>AHHHHHHGSPLPPDITFDSLALIKMHSQSMKK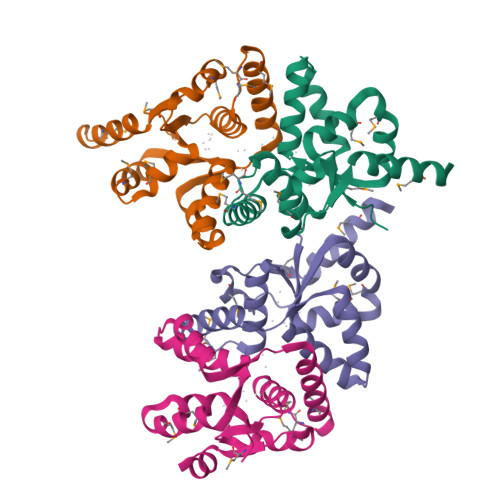ILEITLAKFTVNLSIVTVYRYLTVRAYLKKNIELELDVLKDIYNIVPLNEEIAIKAAQIEADLMRKGMMPDIEDVLTAATAIYTKSLLITDDSKRYEPMRRFGLDTMPLDKFVKEVELMVEKELI[4x]> GSSGSSGMQIGKIIKVSGPLVMAENMSEACIQDMCLVGDLGVIGEIIEMRQDVASIQVY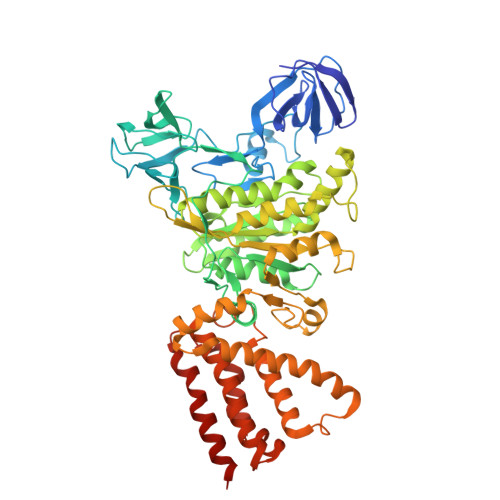EETSGIGPGEPVRSTGEALSVELGPGIISQMFDGIQRPLDTFMEVTQSNFLGRGVQLPALDHEKQWWFEATIEEGTEVSAGDIIGYVDETKIIQHKIMVPNGIKGTVQKIESGSFTIDDPICVIETEQGLKELTMMQKWPVRRGRPIKQKLNPDVPMITGQRVIDTFFPVTKGGAAAVPGPFGAGKTVVQHQIAKWSDVDLVVYVGCGERGNEMTDVVNEFPELIDPNTGESLMERTVLIANTSNMPVAAREASIYTGITIAEYFRDMGYDVAIMADSTSRWAEALREMSGRLEEMPGDEGYPAYLGSRLAEYYERSGRVIALGSDQREGSITAISAVSPSGGDISEPVTQNTLRVVKVFWGLDSSLAQKRHFPSINWIQSYSLYSTEVGRYMDQILQQDWSDMVTEGMRILQEEEQLNEIVRLVGIDSLSDNDRLTLEVAKSIREDYLQQNAFDDVDTFTSREKQFNMLKVILTFGKEARKALSLGAYFNEIMEGTVAVRERISRSKYIPEEELAKISSINEEIKETIQLIVSEGGMTDD> MAGDPNSMTVSHHNASTARFYALRLLPGQEVFSQLHAFVQQNQLRAAWIAGCTGSLTDVALRYAGQEATTSLTGTFEVISLNGTLELTGEHLHLAVSDPYGVMLGGHMMPGCTVRTTLELVIGELPALTFSRQPCAIS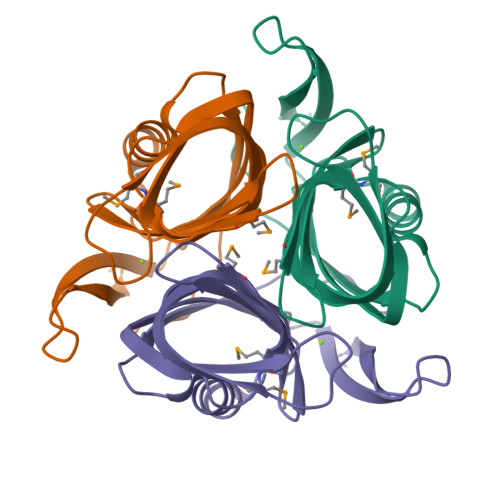GYDELHISSRLEHHHH> GPHMKHPLQNRWALWFFKNDKSKTWQANLRLISKFDTVEDFWALYNHIQLSSNLMPGCDYSLFKDGIEPMWEDEKNKRGGRWLITLNKQQRRSDLDRFWLE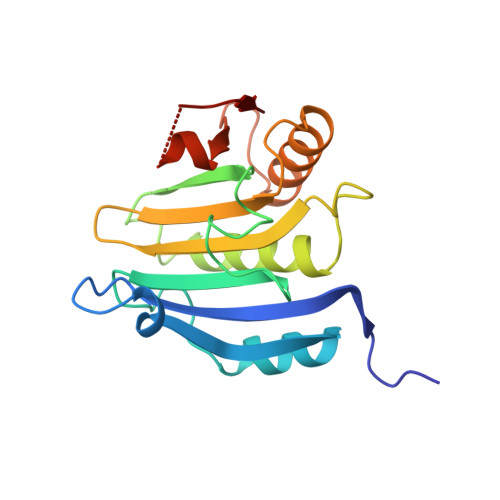TLLCLIGESFDDYSDDVCGAVVNVRAKGDKIAIWTTECENREAVTHIGRVYKERLGLPPKIVIGYQSHADTATKSGSTTKNRFVV> LTPEVGELIEKVRKAHQETFPALCQLGKYTTNNSSEQ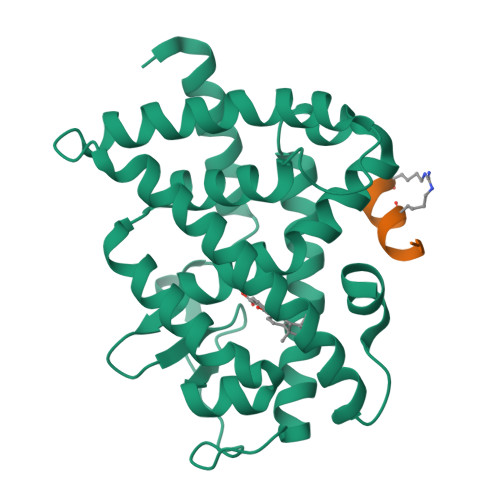RVSLDIDLWDKFSELSTKCIIKTVEFAKQLPGFTTLTIADQITLLKAACLDILILRICTRYTPEQDTMTFSDGLTLNRTQMHNAGFGPLTDLVFAFANQLLPLEMDDAETGLLSAICLICGDRQDLEQPDRVDMLQEPLLEALKVYVRKRRPSRPHMFPKMLMKITDLRSISAKGAERVITLKMEIPGSMPPLIQEMLE;> HKILLRLLRX>SLSSVKDFPKIKAIRSFIIGGVGSGGDYHNVKGGHWLIDSDISTPASKWEQYKKSRTSWGINVLGSFLVEIEATDGTVGFATGFGGPPACWLVHQHFERFLIGADPRNTNLLFEQMYRASMFYGRKGLPIAVISVIDLALWDLLGKVRNEPVYRLIGGATKERLDFYCTGPEPTAAKAMGFWGGKVPLPFCPDDGHEGLRKNVEFLRKHREAVGPDFPIMVDCYMSLNVSYTIELVKACLDLNINWWEECLSPDDTDGFALIKRAHPTVKFTTGEHEYSRYGFRKLVEGRNLDIIQPDVMWLGGLTELLKVAALAAAYDVPVVPHASGPYSYHFQISQPNTPFQEYLANSPDGKSVLPVFGDLFIDEPIPTKGYLTTADLDKPGFGLTINPAARAKLIPSDYLFKVPEIPQNLSTGKEIKSNEQPDKPNGTL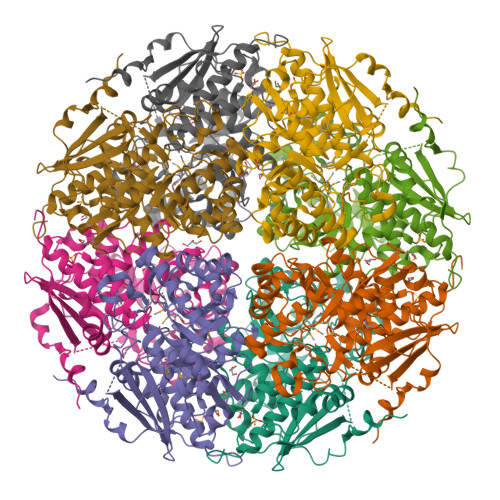DSLAAKVESLTTSTSSEGHHHHHH[8x]>MRSYRAQGPLPGFYHYYPGVPAVVGVRVEERVNFCPAVWNTGLSADPPLFGVSISPKRFTHGLLLKARRFSASFHPFGQKDLVHWLGSHSGREVDKGQAPHFLGHTGVPILEGAYAAYELELLEVHTFGDHDLFVGRVVAVWEEE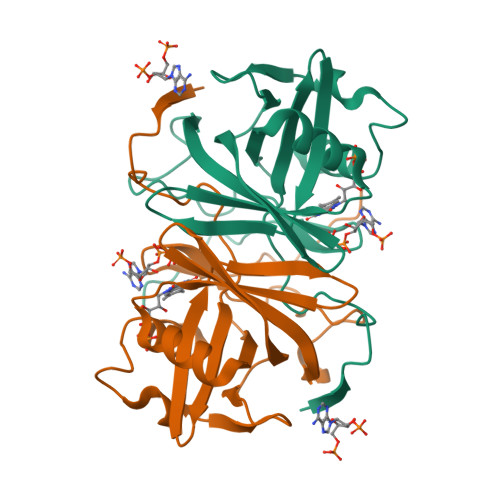GLLDEKGRPKPGLALLYYGKGLYGRPAEETFAP[2x]>[2x]GPGSSKPFTLPILTLGELTNSRFPLPIDVLYTNPNESAIVQCQNGRCTLDGELQGTTQLLPTGICAFRGKVTQQVQDEHRGTHWNMTVTNLNGTPFDPTEDVPAPLGTPDFSGQIYGVISQRNTNTVPGEGNLPANRAHEAVIATYSPKFTPKLGNIQFSTWETQDVSSGQPTKFTPVGLASVDANSHFDQWTLPSYSGALTLNMNLAPSVAPVFPGECLLFFRSFIPLKGGYGNPAIDCLMPQEWVQHL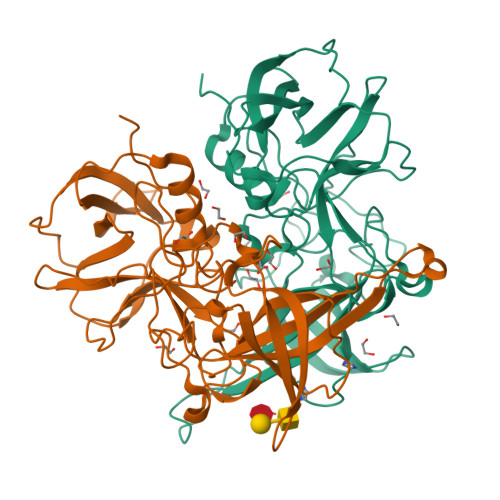YQESAPSLSDVALVRYVNPETGRTLFEAKLHRNGFLTVARNSAGPVVAPTNGYFRFDSWVNQFYTLAPM>[4x]HHHHHHLPNITILATGGTIAGGGDSATKSSYTVGKVGVENLVNAVPQLKDIANVKGEQVVNIGSQDMNDNVWLTLAKKINTDCDKTDGFVITHGTDTMEETAYFLDLTVKCDKPVVMVGAMRPSTSMSADGPFNLYNAVVTAADKASANRGVLVVMNDTVLDGRDVTKTNTTDVATFKSVNYGPLGYIHNGKIDYQRTPARKHTSDTPFDVSKLNELPKVGIVYNYANASDLPAKAL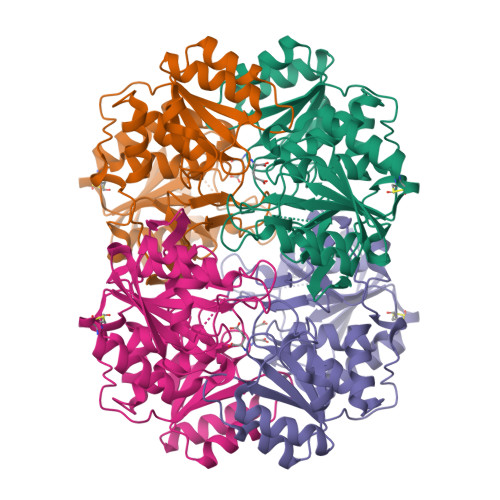VDAGYDGIVSAGVGNGNLYKSVFDTLATAAKTGTAVVRSSRVPTGATTQDAEVDDAKYGFVASGTLNPQKARVLLQLALTQTKDPQQIQQIFNQY>[3x]MQQLQNVIESAFERRADITPANVDTVTREAVNQVIGLLDSGALRVAEKIDGQWVTHQWLKKAVLLSFRINDNKVMDGAETRYYDKVPMKFADYDEARFQKEGFRVVPPATVRQGAFIARNTVLMPSYVNIGAYVDEGTMVDTWATVGSCAQIGKNVHLSGGVGIGGVLEPLQANPTIIEDNCFIGARSEVVEGVIVEEGSV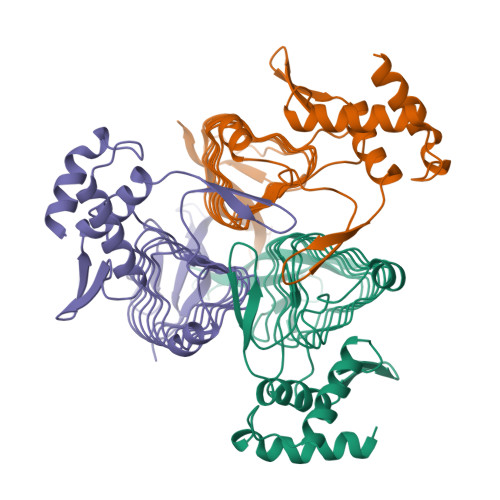ISMGVYLGQSTRIYDRETGEIHYGRVPAGSVVVSGNLPSKDGSYSLYCAVIVKKVDAK>MQDRGNTVTIDFMSADGIVPGRTPVRYQGVEVGTVQDISLSDDLRKIEVKVSIKSDMKDALREETQFWLVTPKASLAGVSGLDALVGGNYIGMMPGKGKEQDHFVALDTQPKYRLDNGDLMIHLQAPDLGSLNSGSLVYFRKIPVGKVYDYAINPNKQGVVIDVLIERRFTDLVKKGSRFWNVSGVDANVSISGAKVKLESLAALVNGAIAFDSPEESKPAEAEDTFGLYEDLAHSQRGVIIKLELPSGAGLTADSTPLMYQGLEVGQLTKLDLNPGGKVTGEMTVDPSVVTLLRENTRIELRNPKLSLSDANLSALLTGKTFELVPGDGEPRKEFVVVPGEKALLHEPDVLTLTLTAPESYGIDAGQPLILHGVQVGQVIDRKLTSKGVTFTVAIEPQHRELVKGDSKFVVNSRVDVKVGLDGVEFLGASASEWINGGIRILPGDKGEMKASYPLYANLEKALENSLSDLPTTTVSLSAETLPDVQAGSVVLYRKFEVGEVITVRPRANAFDIDLHIKPEYRNLLTSNSVFWAEGGAKVQLNGSGLTVQASPLSRALKGAISFDNLSGASASQRKGDKRILYASETAARAVGLSIIVEAPEAGSLGIGTPVLFRGLEVGTVTGMTLGTLSDRVMIAMRISKRYQHLVRNNSVFWLASGYSLDFGLTGGVVKTGTFNQFIRGGIAFATPPGTPLAPKAQEGKHFLLQESEPKEWREW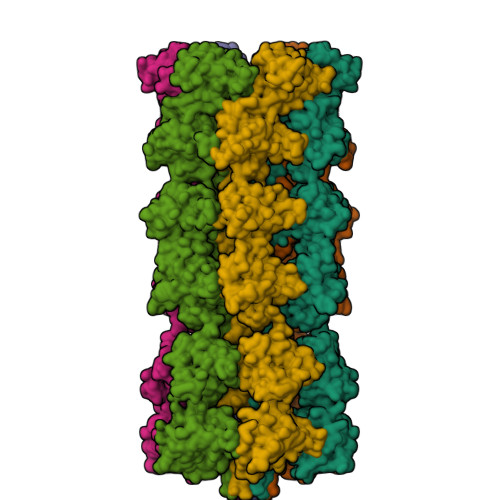GTALPKGETHHHHHH[6x]>[2x]SNAERKYSTFYEQRAT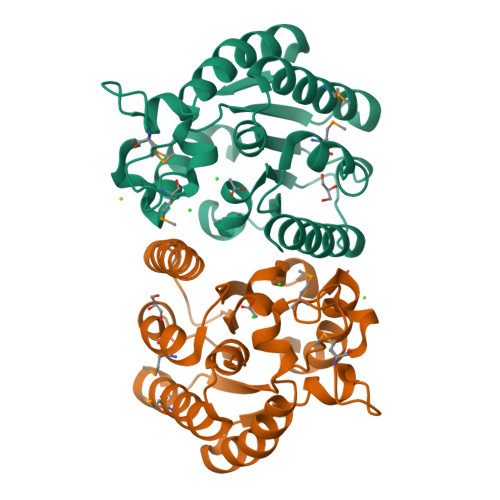LFEELPVTSKDIIFLGNSITNGCEWAELFQNKNVKNRGISGDICMGVYDRLDPIVKGKPAKIFLLIGINDVSRGTSADKIISEISMIVRKIKQESPKTKLYLQSVLPVNDCYGMFNGHTSRWQVVKQINDLLEPLAVKEGVAYIDLYSHFVEKETGKMNPVYTNDGLHLLGKGYLLWRDIVKPYVD Urease is a nickel containing metalloenzyme that hydrolyses urea into ammonia. Four urease accessory proteins—UreE, UreF, UreG, and UreH (UreH is an ortholog of UreD found in other species)—participate in the regulation of nickel delivery and urease maturation. UreG is a SIMIBI (after signal recognition particle, MinD, and BioD) class GTPase involved in the regulation of nickel delivery. The interactions between urease and its accessory proteins were further supported by yeast-two-hybrid and tandem affinity purification. It was hypothesized that the UreG/UreF/UreH complex is responsible for delivery of nickel ions into the urease active site and the formation of the preactivation complex is a critical step involved in urease maturation.

To gain insight into the urease maturation process, we determined the structure of the UreG/UreF/UreH complex in its GDP-bound state to 2.35 Å resolution using X-ray crystallography. The asymmetric unit contains two copies of each of UreF, UreH, and UreG, related by 2-fold symmetry, forming a dimer of heterotrimers. The UreG/UreF/UreH complex structure represents the first known structure of UreG. The topology of UreG is characteristic of SIMIBI class GTPases containing the canonical G1 to G5 motif for guanine nucleotide recognition. Two GDP ligands are sandwiched between two UreG protomers. UreG contains an invariant Cys66-Pro67-His68 metal binding motif, substitution of which abolishes the metal binding properties of UreG. This metal binding motif is found at the dimer interface between two UreG protomers. Cys66 and His68 from each protomer are arranged in a symmetric formation that could potentially bind a metal ion at the interface. The crystal structure also showed that UreG interacts strictly with UreF only, leading to an overall structure resembling that of an inverted-T shape. Each UreG protomer makes extensive contacts with both protomers of UreF.

>MDKGKSVKSTEKSVGMPPKTPKTDNNAHVDNEFLILQVNDAVFPIGSYTHSFGLETYIQQKKVTNKESALEYLKANLSSQFLYTEMLSLKLTYESALQQDLKKILGVEEVIMLSTSPMELRLANQKLGNRFIKTLQAMNELDMGEFFNAYAQKTKDPTHATSYGVFAASLGIELKKALRHYLYAQTSNMVINCVKSVPLSQNDGQKILLSLQSPFNQLIEKTLELDESHLCTASVQNDIKAMQHESLYSRLYMS[2x];>[2x]MNTYAQESKLRLKTKIGADGRCVIEDNFFTPPFKLMAPFYPKDDLAEIMLLAVSPGMMRGDAQDVQLNIGPNCKLRITSQSFEKIHNTEDGFASRDMHIVVGENAFLDFAPFPLIPFENAHFKGNTTISLRSSSQLLYSEIIVAGRVARNELFKFNRLHTKISILQDEKPIYYDNTILDPKTTDLNNMCMFDGYTHYLNLVLVNCPIELSGVRECIEESEGVDGAVSETASSHLCVKALAKGSEPLLHLREKIARLVTQTTTQKV;>[2x]MVKIGVCGPVGSGKTALIEALTRHMSKDYDMAVITNDIYTKEDAEFMCKNSVMPRERIIGVETGGCPHTAIREDASMNLEAVEEMHGRFPNLELLLIESGGDNLSATFNPELADFTIFVIDVAEGDKIPRKGGPGITRSDLLVINKIDLAPYVGADLKVMERDSKKMRGEKPFIFTNIRAKEGLDDVIAWIKRNALLED4-({[(3R,5R,6S)-1-[(1S)-2-(tert-butylsulfonyl)-1-cyclopropylethyl]-6-(4-chloro-3-fluorophenyl)-5-(3-chlorophenyl)-3-methyl-2-oxopiperidin-3-yl]acetyl}amino)-2-methoxybenzoic 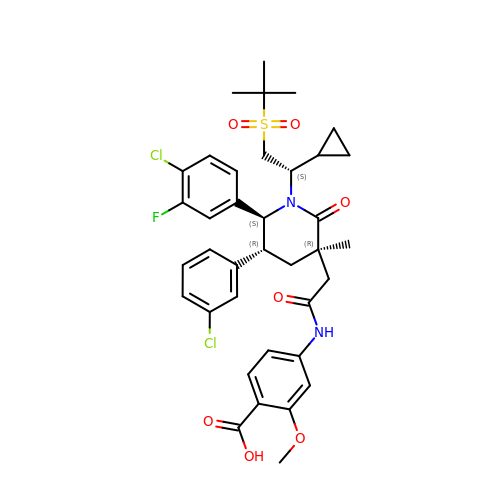acid | C37 H41 Cl2 F N2 O7 S | QGOICCMBEDDFCI-NXQGQTBASA-N>[2x]MPKKTIYFGAGWFTDRQNKAYKEAMEALK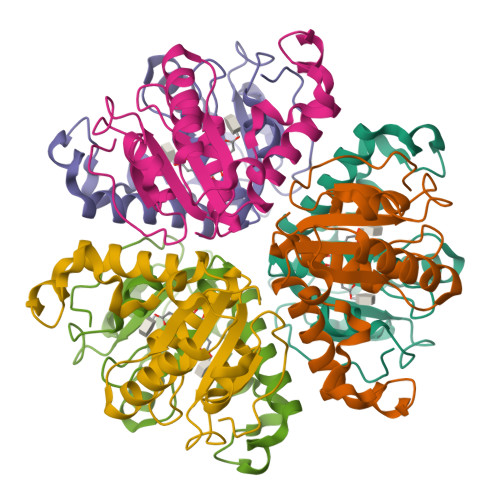ENPTIDLENSYVPLDNQYKGIRVDEHPEYLHDKVWATATYNNDLNGIKTNDIMLGVYIPDEEDVGLGMELGYALSQGKYVLLVIPDEDYGKPINLMSWGVSDNVIKMSQLKDFNFNKPRFDFYEGAVY> SDVCPLTLGIETVGGVMTKLIPRNTVVPTKKSQIFSTASDNQ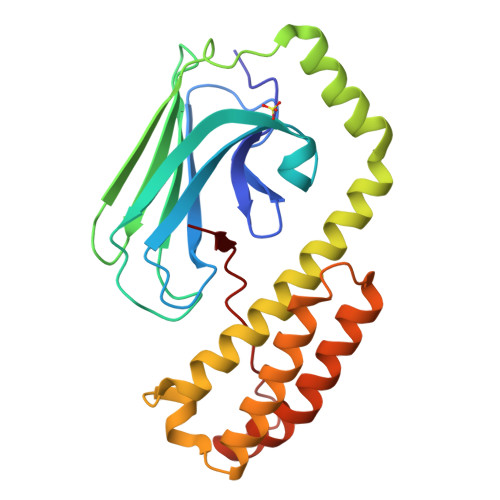PTVTIKVYEGERPLTKDNHLLGTFDLTGIPPAPRGVPQIEVTFEIDVNGILRVTAEDKGTGNKNKITITNDQNRLTPEEIERMVNDAEKFAEEDKKLKERIDTRNELESYAYSLKNQIGDKEKLGGKLSSEDKETMEKAVEEKIEWLESHQDADIEDFKAKKKELEEIVQPIISKLYGSENLYFQGSNRLLLTG>MTRYTAPTQDIQYLLHDVLDVANDPTPGYAEL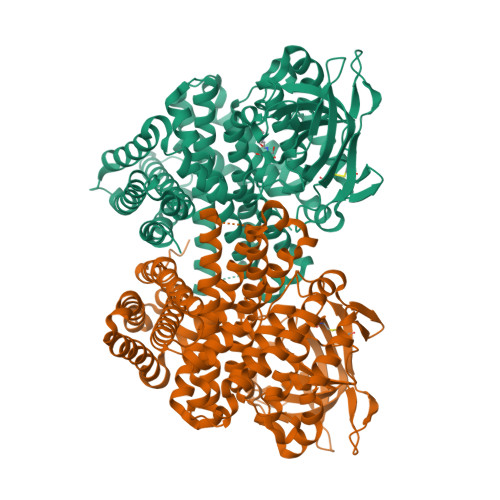EPDFTSAVLEEAGKIAGEVLHPLNAVGDQEGCVLENGVVRPPKGFKEAFDQVREGGWTALDLPEQYGGQNMPYLLGTAVGEMFSGANQAFTMYQGLTHGAASAILVHGTDQQKDTYLPKMFSCDWTGTMNLTEPHCGTDLGLMRSKAVPQDDGSYAISGQKIFISAGEHDMAENIIHLVLAKIPGGPEGIKGVSLFIVPKFLVKEDGSLGERNGVKCSKIEEKMGIHGNSTCVMDYDGAKGWLLGEEHKGMRAMFTMMNEARIGVGMQGLAQAEVAYQNALDYARDRLQGRSVTGVENPDGPADPLIVHPDIRRNLLDQKSFIEGARAFLLWGAQMIDRAERGKDEAAHGMVSLLTPVIKGFLTDEGYDMTVQAQQVYGGHGYIEETGMSQFTRDARIAMIYEGANGVQALDLVGRKLAQDGGKHVMAFFDLVKGFIKEAGTDGAMAEFTEPLKSASKDLQSAGMFFMQNGMKNPNAALAGSYDFMHLFGHVCLGLMWGRMAEASLKALAEGRGDANFHETKLATARFYMTRRLPATKLHLARIESGADPVMALDADRF[2x]>MGAHSKEMAPLMGKRTTAPGGNPVVLTEKRPADLTPTKKSAHFFLEIEGFEPNPTVTKTSPPIFSKPMDSNIRQCLSGNCDDMDSPQSPQDDVTETPSNPNSPSANLAKEEQRQKKKRLKKRIFAAVSEGCVEELRELLQDLQDLCRRRRGLDVPDFLMHKLTASDTGKTCLMKALLNINPNTKEIVRILLAFAEENDILDRFINAEYTEEAYEGQTALNIAIERRQGDITAVLIAAGADVNAHAKGVFFNPKYQHEGFYFGETPLALAACTNQPEIVQLLMENEQTDITSQDSRGNNILHALVTVAEDFKTQNDFVKRMYDMILLRSGNWELETMRNNDGLTPLQLAAKMGKAEILKYILSREIKEKPLRSLSRKFTDWAYGPVSSSLYDLTNVDTTTDNSVLEIIVYNTNIDNRHEMLTLEPLHTLLHTKWKKFAKYMFFLSFCFYFFYNITLTLVSYYRPREDEDLPHPLALTHKMSWLQLLGRMFVLIWATCISVKEGIAIFLLRPSDLQSILSDAWFHFVFFVQAVLVILSVFLYLFAYKEYLACLVLAMALGWANMLAYTRGFQSMGMYSVMIQKVILHDVLKFLFVYILFLLGFGVALASLIEKCSKDKKDCSSYGSFSDAVLELFKLTIGLGDLNIQQNSTYPILFLFLLITYVILTFVLLLNMLIALMGETVENVSKESERIWRLQRARTILEFEKMLPEWLRSRFRMGELCKVADEDFRLCLRINEVKWTEWKTHVSFLNEDPGPIRRT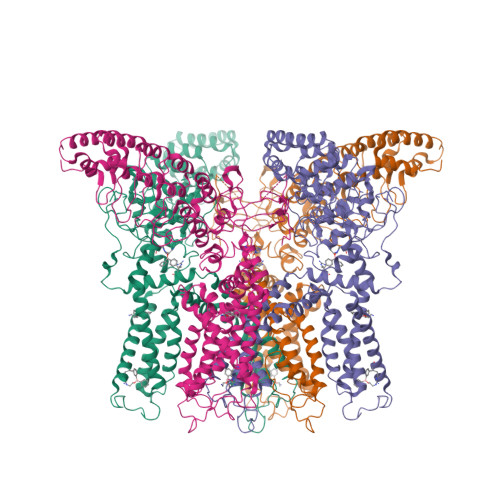ADLNKIQDSSRSNSKTTLYAFDELDEFPETSV[4x]>[10x]MSIVTKSIVNADAEARYLSPGELDRIKAFVTGGAARLRIAETLTGSRETIVKQAGDRLFQKRPDIVSPGGNAYGEEMTATCLRDMDYYLRLVTYGVVSGDVTPIEEIGLVGVREMYRSLGTPIEAVAQSVREMKEVASGLMSSDDAAEASAYFDFVIGKMS;>[11x]MQDAITAVINSADVQGKYLDGAAMDKLKSYFASGELRVRAASVISANAATIVKEAVAKSLLYSDVTRPGGNMYTTRRYAACIRDLDYYLRYATYAMLAGDASILDERVLNGLKETYNSLGVPISSTVQAIQAIKEVTASLVGADAGKEMGVYLDYICSGLS;> MSVVSQVILQADDQLRYPTSGELKGIQAFLTTGAQRIRIAETLAENEKKIVDQAQKQLFKKHPEYRAPGGNAYGQRQYNQCLRDYGWYLRLVTYGVLAGNKEPIETTGLIGVKEMYNSLNVPVPGMVDAVTVLKDAALGLLSAEDANETAPYFDYIIQFMS;> MRDAVTTLIKNYDLTGRYLDRNAMDELKAYFESGSARIAAAAMINANSATIVKRAAAQLFEEIPELIRPSGNAYTTRRFSACLRDMDYYLRYASYALIAADNNVLDERVLQGLRETYNSLGVPIGPTVRGIQIMKEMIEAMAEDSSLNSTDFIASPFDHMTRELSELSV;>MRMFRITACVPSQTRIRTQRELQNTYFTKLVPYDNWFREQQRIMKMGGKIVKVELATGRPGTNAGLA[2x];> MSVKASGGSSLARPQLYQTVPVSAISQAEQQDRFLEGSELNELTAYFQSGALRLEIAETLTQNADLIVSRAANRIFTGGSPLS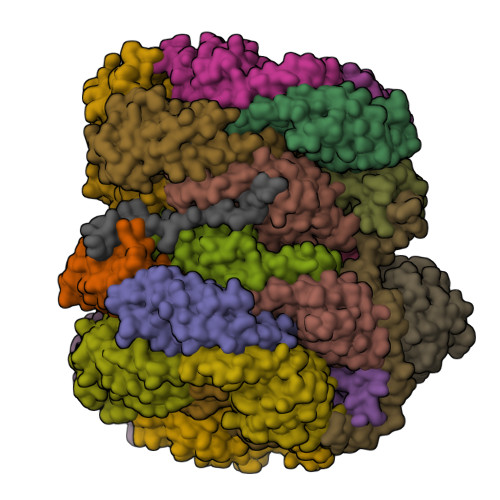YLEKPVERQPALVGASSDSRNGSVTYAESNGSGGLFGGLRSVFSSTGPIPPGFRPINIARYGPSNMQKSLRDMSWFLRYTTYAIVAGDPNIIVVNTRGLKEVIENACSIDATIVAIQEMRAASADYFRNNAQAKEIVLQYFDILLSEFKAPTPANKVRQGPSNDIQGLELPQSYFNAAAKRQKYAMKPGLSALEKNAVIKAAYRQIFERDITKAYSQSISYLESQVRNGDISMKEFVRRLAKSPLYRKQFFEPFINSRALELAFRHILGRGPSSREEVQKYFSIVSSGGLPALVDALVDSQEYADYFGEETVPYLRGLGVEAQECRNWGMQQDLFSYSAPFRKVPQFITTFAQYDRPLPDQHVYGSGNDPLEIQFGAIFPKETRNPSKRPAPFNKDTKRILIHRGPAVNNQVGNPSAVGEFPGSLGAKVFRLNGGLPGAKVGKNTGTSVKFGESSTQALIRAAYRQVFGRDLYEGQRLSVAEIQLENGDISVREFIKRLAKSELFLKLYWAPHYVCKAIEYMHRRLLGRPTYGRQEMNQYFDIASKQGFYAVVEAMIDSKEYSDAFGEDTVPYERYLTPGGLQMRSARVGSLREDIGQRVDKEVTPRFVELGQVSAIRTEPEIAYRSNQGVTRQRQQTKVFKLVSTYDKVAVKNAIRAAYRQVFERDLEPYIINSEFTALESKLSNNEINVKEFIEGLGTSELYMKEFYAPYPNTKVIEMGTKHFLGRAPLNQKEIQQYNQILASQGLKAFIGAMVNGMEYLQTFGEDTVPYRRFPTLPAANFPNTERLYNKLTKQDKELVVPSFTPVVKVGG;> MALPLLNYAPKSQNVRVEGYEIGSEEKPVVFTTENILSSSDMDNLIEAAYRQIFFHAFKWDREKVLESQLRNGQITVRDFVRGLLLSNTFRNSFYEKNSNYRFVEHCVQKILGRDVYSEREKIAWSIVVATKGYQGLIDDLLNSDEYLNNFGYDTVPYQRRRNLPGREAGELPFNIKSPRYDAYHRRQLGFPQIVWQNEVRRFIPQEKKLTAGNPMNFLGMARSINPAANTIPKVSAQNINIEASVPRR;> MPFTIDSARGIFPNTLAADVVPATIARFSQLNAEDQLALIWFAYLEMGKTLTIAAPGAASMQLAENALKEIQAMGPLQQTQAMCDLANRADTPLCRTYASWSPNIKLGFWYRLGELMEQGFVAPIPAGYQLSANANAVLATIQGLESGQQITVLRNAVVDMGFTAGKDGKRIAEPVVPPQDTASRTKVSIEGVTNATVLNYMDNLNANDFDTLIELFTSDGALQPPFQRPIVGKENVLRFFREECQNLKLIPERGVTEPAEDGFTQIKVTGKVQTPWFGGNVGMNIAWRFLLNPEGKIFFVAIDLLASPKELLNFAR;> MLKKLFGAKKEFYVQLDESQAPAQVEEADVAIVKSEVAPVEKPAPTTSKKTSIKKKSATKAAAPVETPASAPVAPAPKAKVDPSQVAFASGDPIPQNVARRTPGPSLNRFKEMARQVKVKR> MIVSDIEANALLESVTKFHCGVIYDYSTAEYVSYRPSDFGAYLDALEAEVARGGLIVFHNGHKYDVPALTKLAKLQLNREFHLPRENCIDTLVLSRLIHSNLKDTDMGLLRSGKLPGALEAWGYRL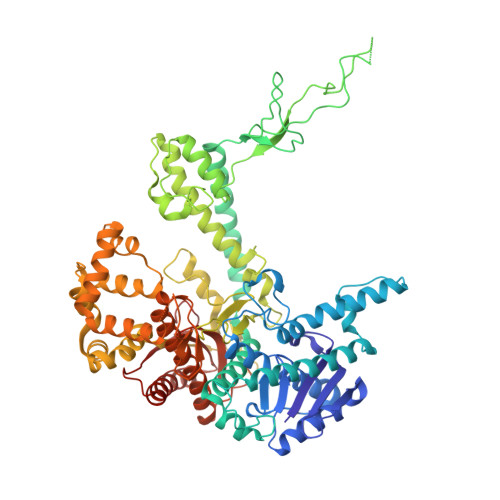GEMKGEYKDDFKRMLEEQGEEYVDGMEWWNFNEEMMDYNVQDVVVTKALLEKLLSDKHYFPPEIDFTDVGYTTFWSESLEAVDIEHRAAWLLAKQERNGFPFDTKAIEELYVELAARRSELLRKLTETFGSWYQPKGGTEMFCHPRTGKPLPKYPRIKTPKVGGIFKKPKNKAQREGREPCELDTREYVAGAPYTPVEHVVFNPSSRDHIQKKLQEAGWVPTKYTDKGAPVVDDEVLEGVRVDDPEKQAAIDLIKEYLMIQKRIGQSAEGDKAWLRYVAEDGKIHGSVNPNGAVTGRATHAFPNLAQIPGVRSPYGEQCRAAFGAEHHLDGITGKPWVQAGIDASGLELRCLAHFMARFDNGEYAHEILNGDIHTKNQIAAELPTRDNAKTFIYGFLYGAGDEKIGQIVGAGKERGKELKKKFLENTPAIAALRESIQQTLVESSQWVAGEQQVKWKRRWIKGLDGRKVHVRSPHAALNTLLQSAGALICKLWIIKTEEMLVEKGLKHGWDGDFAYMAWVHDEIQVGCRTEEIAQVVIETAQEAMRWVGDHWNFRCLLDTEGKMGPNWAICH(2Z,3aR,5R,6S,7R,7aR)-2-(ethylimino)-5-(hydroxymethyl)hexahydro-3aH-pyrano[3,2-d][1,3]thiazole-6,7-diol | C9 H16 N2 O4 S | 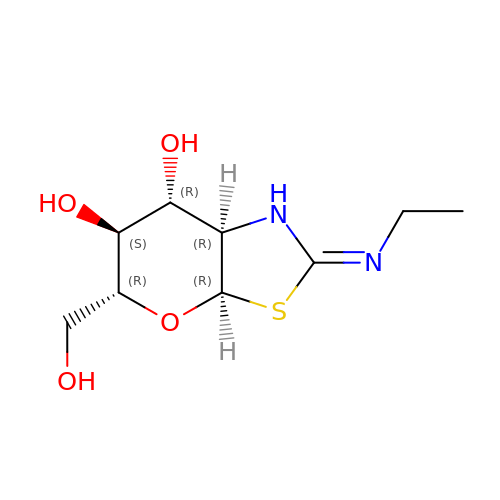PPAIMZHKIXDJRN-FMDGEEDCSA-N> MHCRSHEEVNTELKAQIMKEIRKPGRKYERIFTLLKHVQGSLQTRLIFLQNVIKEASRFKKRMLIEQLE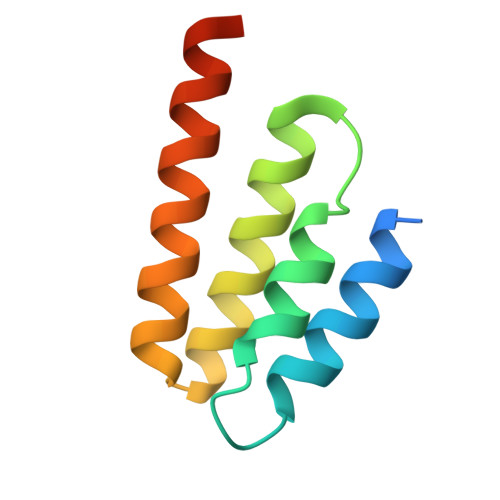NFLDEIHRRANQINHINSN> MTNESILESYSGVTPERKKSRMPAKLDWWQSATGLFLG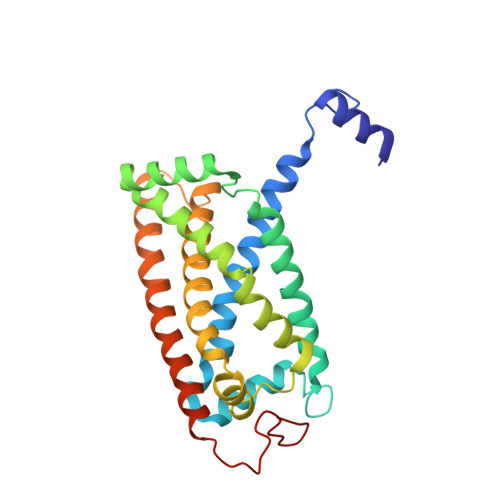LFMIGHMFFVSTILLGDNVMLWVTKKFQLDFIFEGGKPIVVSFLAAFVFAVFIAHAFLAMRKFPINYRQYLTFKTHKDLMRHGDTTLWWIQAMTGFAMFFLGSVHLYIMMTQPQTIGPVSSSFRMVSEWMWPLYLVLLFAVELHGSVGLYRLAVKWGWFDGETPDKTRANLKKLKTLMSAFLIVLGLLTFGAYVKKGLEQTDPNIDYKYFDYKRTHHR3-(CYCLOPENTYLOXY)-N-(3,5-DICHLOROPYRIDIN-4-YL)-4-METHOXYBENZAMIDE 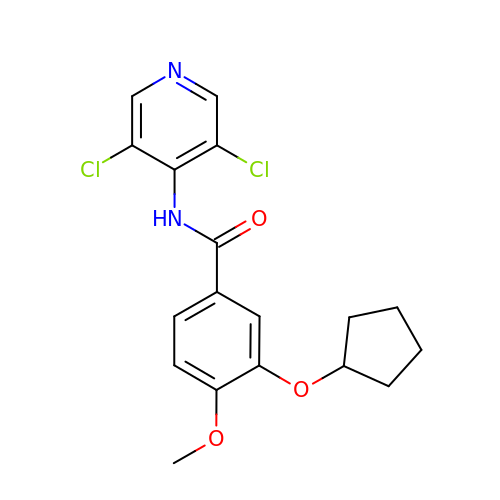| C18 H18 Cl2 N2 O3 | RRRUXBQSQLKHEL-UHFFFAOYSA-N For the levan utilisation system, the cell surface components are Bt1760 (a GH32 endo-levanase), Bt1761 (a surface glycan-binding protein; SGBP), Bt1762 (SusD) and Bt1763 (SusC)15,19,24. SusC proteins are unique among TBDTs in that they are tightly associated with a SusD substrate-binding lipoprotein15–17. Recently, we showed that SusCD complexes mediate substrate uptake via a “pedal bin” mechanism. The SusC transporter forms the barrel of the bin, while SusD sits on top of the barrel, opening and closing like a lid to facilitate substrate binding.

To visualise potential different conformational states, we used single-particle cryo-EM on detergent-solubilised apo-Bt1762-63. Strikingly, several distinct conformations of the SusC2D2 complex are present in a single dataset, and after further classification steps, three dominant states were identified. Following three-dimensional (3D) reconstruction, electron density maps were obtained at resolutions allowing rigid body placement and refinement of individual protomers. This yielded structures corresponding to the three possible combinations of open and closed dimeric transporters: OO (3.9 Å), OC (4.7 Å) and CC (4.2 Å). With the exception of a few Bt1763 loops (L6 and L7) and the Bt1762 segment following the lipid anchor that serves as a pivot around which Bt1762 moves upon lid opening, the conformational changes between the three states correspond to rigid body movements of Bt1762. Interestingly, the presence of the plug domain in the interior of the Bt1763 barrel in solution is strictly correlated with the open vs. closed state of the transporter; only open states contain a plug domain, regardless of the state of the SusC2D2 dimer. Mutational studies in vivo provide insights into the key structural features of the SusCD apparatus and cryo-electron microscopy (EM) of the intact SusC2D2 complex reveals several distinct states of the transporter, that is, open-open (OO), open-closed (OC) and closed-closed (CC). These structures directly visualise the dynamics of the pedal bin mechanism and suggest that the individual SusCD complexes function independently of each other.

>MKKIIYIATIGITLLTTSCDDFLDRQVPQGIVTGDQIASPEYVDNLVISAYAIWATGDDINSSFSLWNYDVRSDDCYKGGSGTEDGGVFNALEISKGINTTDWNINDIWKRLYQCITRANTALQSLDQMDEKTYPLKNQRIAEMRFLRGHAHFMLKQLFKKIVIVNDENMEPDAYNELSNTTYTNDEQWQKIADDFQFAYDNLPEVQIEKGRPAQAAAAAYLAKTYLYKAYRQDGADNALTGINEEDLKQVVKYTDPLIMAKGGYGLETDYSMNFLPQYENGAESVWAIQYSINDGTYNGNLNWGMGLTTPQILGCCDFHKPSQNLVNAFKTDSQGKPLFSTYDNENYEVATDNVDPRLFHTVGMPGFPYKYNEGYIIQKNDDWSRSKGLYGYYVSLKENVDPDCDCLKKGSYWASSLNHIVIRYADVLLMRAEALIQLNDGRITDAISLINEVRSRAAGSTMLIFNYKEDYGVNFKVTPYDLKAYAQDEAMKMLKWERRVEFGMESSRFFDLVRWGEAKDVINAYYVTEASRCSIYKNAGFTENKNEYLPVPFEQISASNGNYTQNFGWAAAAHHHHHH[2x];>MPGIMKNKKLLCSVCFLFAFMSALWGQNITVKGNVTSKTDGQPIIGASVVETTATTNGTITDFDGNFTLSVPVNSTLKITYIGYKPVTVKAAAIVNVLLEEDTQMVDEVVVTGYTTQRKADLTGAVSVVKVDEIQKQGENNPVKALQGRVPGMNITADGNPSGSATVRIRGIGTLNNNDPLYIIDGVPTKAGMHELNGNDIESIQVLKDAASASIYGSRAANGVIIITTKQGKKGQIKINFDASVSASMYQSKMNVLNTEQYGRAMWQAYVNDGENPNGNALGYAYNWGYNADGNPVLYGMTLSKYLDSKNTMPVADTDWFDEITRTGVIQQYNLSVSNGSEKGSSFFSLGYYKNLGVIKDTDFDRFSARMNSDYKLIDDILTIGQHFTLNRTSEVQAPGGIIETALDIPSAIPVYASDGSWGGPVGGWPDRRNPRAVLEYNKDNRYTYWRMFGDAYVNLTPFKGFNLRSTFGLDYANKQARYFTYPYQEGTQTNNGKSAVEAKQEHWTKWMWNAIATYQLEVGKHRGDVMIGMELNREDDSHFSGYKEDFSILTPDYMWPDAGSGTAQAYGAGEGYSLVSFFGKMNYSYADRYLLSLTLRRDGSSRFGKNHRYATFPSVSLGWRITQENFMKELTWLDDLKLRASWGQTGNQEISNLARYTIYAPNYGTTDSFGGQSYGTAYDITGSNGGGVLPSGFKRNQIGNDNIKWETTTQTNVGIDFSLFKQSLYGSLEYYYKKATDILTEMAGVGVLGEGGSRWINSGAMKNQGFEFNLGYRNKTAFGLTYDLNGNISTYRNEILELPETVAANGKFGGNGVKSVVGHTYGAQVGYIADGIFKSQDEVDNHATQEGAAVGRIRYRDIDHNGVIDERDQNWIYDPTPSFSYGLNIYLEYKNFDLTMFWQGVQGVDIISDVKKKSDFWSASNVGFLNKGTRLLNAWSPTNPNSDIPALTRSDTNNEQRVSTYFVENGSFLKLRNIQLGYTVPAVISKKMRMDRLRFYCSAQNLLTIKSKNFTGEDPENPNFSYPIPVNITFGLNIGF[2x]> GSHMTTQTTPAHIAMFSIAAHGHVNPSLEVIRELVARGHRVTYAIPPVFADKVAATGARPVLYHSTLPGPDADPEAWGSTLLDNVEPFLNDAIQALPQLADAYADDIPDLVLHDITSYPARVLARRWGVPAVSLSPNLVAWKGYEEEVAEPMWREPRQTERGRAYYARFEAWLKENGITEHPDTFASHPPRSLVLIPKALQPHADRVDEDVYTFVGACQGDRAEEGGWQRPAGAEKVVLVSLGSAFTKQPAFYRECVRAFGN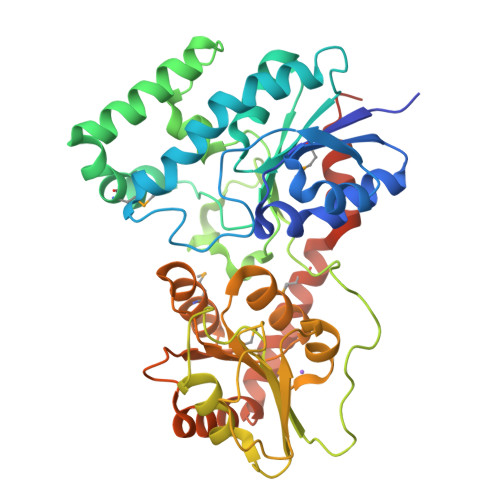LPGWHLVLQIGRKVTPAELGELPDNVEVHDWVPQLAILRQADLFVTHAGAGGSQEGLATATPMIAVPQAVDQFGNADMLQGLGVARKLATEEATADLLRETALALVDDPEVARRLRRIQAEMAQEGGTRRAADLIEAELPARHERQEPVGDRPNGG> IVGGKVCPKGECPWQVLLLVNGAQLCGGTLINTIWVVSAAHCFDKIKNWRNLIAVLGEHDLSEHDGDEQSRRVAQVIIPSTYVPGTTNHDIALLRLHQPVVLTDHVVPLCLPERTFSERTLAFVRFSLVSGWGQLLDRGATALELMVLNVPRLMTQDCLQQSRKVGDSPNITEYMFCAGYSDGSKDSCKGDSGGPHATHYRGTWYLTGIVSWGQGCATVGHFGVYTRVSQYIEWLQKLMRSEPRPGVLLRAPFP;> ANAFLEELRPGSLERECKEEQCSFEEAREIFKDAERTKLFWISYSDGDQCASSPCQNGGSCKDQLQSYICFCLPAFEGRNCETHKDDQLICVNENGGCEQYCSDHTGTKRSCRCHEGYSLLADGVSCTPTVEY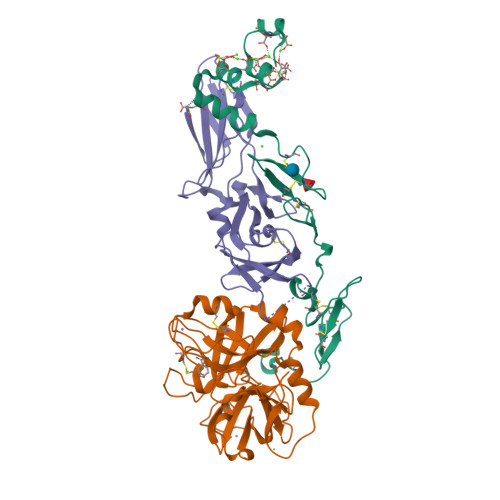PCGKIPILE;> ATVAAYNLTWKSTNFKTILEWEPKPVNQVYTVQISTKSGDWKSKCFYTTDTECDLTDEIVKDVKQTYLARVFSYPAGNVESTGSAGEPLYENSPEFTPYLETNLGQPTIQSFEQVGTKVNVTVEDERTLVRRNNTFLSLRDVFGKDLIYTLYYWKSSSSGKKTAKTNTNEFLIDVDKGENYCFSVQAVIPSRTVNRKSTDSPVECM>[4x]DIISVALKRHSTKAFDASKKLTAEEAEKIKTLLQYSPSSTNSQPWHFIVASTEEGKARVAKSAAG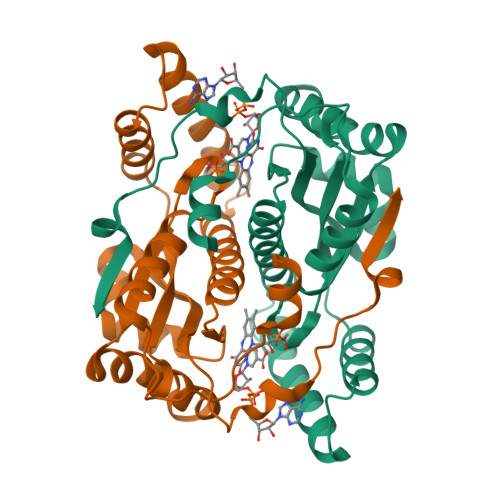TYVFNERKMLDASHVVVFCAKTAMDDAWLERVVDQEEADGRFNTPEAKAANHKGRTYFADMHRVDLKDDDQWMAKQVYLNVGNFLLGVGAMGLDAVPIEGFDAAILDEEFGLKEKGFTSLVVVPVGHHSVEDFNATLPKSRLPLSTIVTEC>GPMPGKKVVARVAEARAEDVGKRVVRVDKAERAKVGVKVGDVV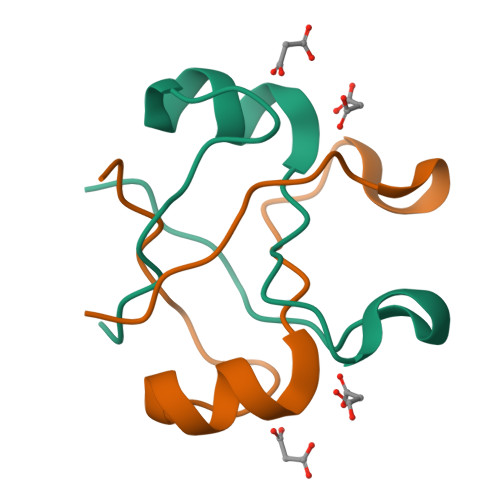EVKKV[4x]>[2x]MKLAARVESVSPSMTLIIDAKAKAMKAEGIDVCSFSAGEPDFNTPKHIVEAAKAALEQGKTRYGPAAGEPRLREAIAQKLQRDNGLCY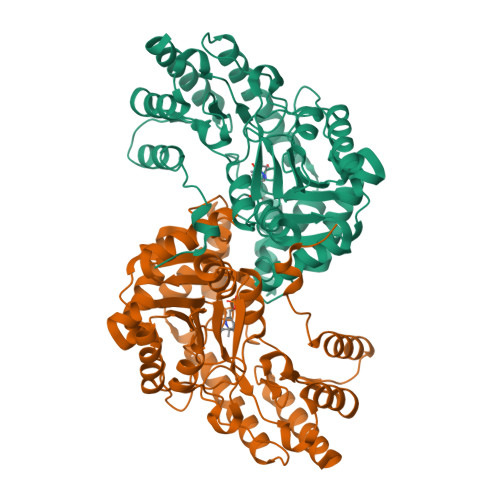GADNILVTNGGKQSIFNLMLAMIEPGDEVIIPAPFWVSYPEMVKLAEGTPVILPTTVETQFKVSPEQIRQAITPKTKLLVFNTPSNPTGMVYTPDEVRAIAQVAVEAGLWVLSDEIYEKILYDDAQHLSIGAASPEAYERSVVCSGFAKTYAMTGWRVGFLAGPVPLVKAATKIQGHSTSNVCTFAQYGAIAAYENSQDCVQEMLAAFAERRRYMLDALNAMPGLECPKPDGAFYMFPSIAKTGRSSLDFCSELLDQHQVATVPGAAFGADDCIRLSYATDLDTIKRGMERLEKFLHGIL> MRDSTECQRIIRRGVNCLMLPKGMQRSSQNRSKWDKTMDLFVWSVEWILCPMQEKGEKKELFKHVSHRIKETDFLVQGMGKNVFQKCCEFYRLAGTSSCIEGEDGSETKEERTQILQKSGLKFYTKTFPYNTTHIMDSKKLVELAIHEKCIGELLKNTTVIEFPTIFVAMTEADLPEGYEVLH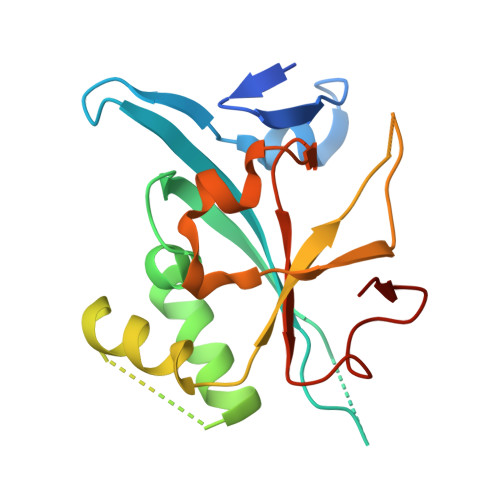QE>SNAMGTIKIVTDSSITIEPELIKALDIT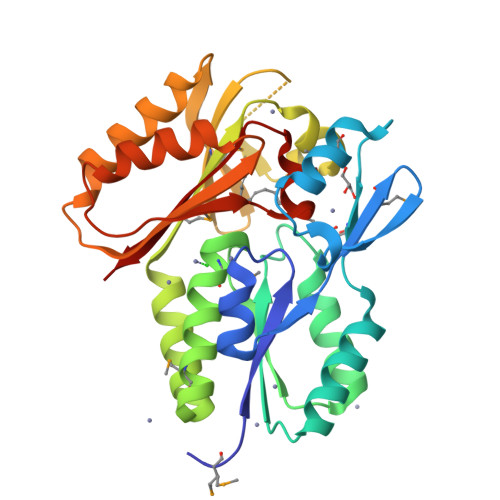VVPLSVMIDSKLYSDNDLKEEGHFLSLMKASKSLPKTSQPPVGLFAETYENLVKKGVTDIVAIHLSPALSGTIEASRQGAEIAEAPVTVLDSGFTDQAMKFQVVEAAKMAKAGASLNEILAAVQAIKSKTELYIGVSTLENLVKGGRIGRVTGVLSSLLNVKVVMALKNDELKTLVKGRGNKTFTKWLDSYLAKNSHRPIAEIAISYAGEASLALTLKERIAAYYNHSISVLETGSIIQTHTGEGAFAVMVRYE[2x]> MDSKHQCVKLNDGHFMPVLGFGTYAPPEVPRSKALEVTKLAIEAGFRHIDSAHLYNNEEQVGLAIRSKIADGSVKREDIFYTSKLWSTFHRPELVRPALENSLKKAQLDYVDLYLIHSPMSLKPGEELSPTDENGKVIFDIVDLCTTWEAMEKCKDAGLAKSIGVSNFNRRQLEMILNKPGLKYKPVCNQVECHPYFNRSKLLDFCKSKDIVLVAYSALGSQRDKRWVDPNSPVLLEDPVLCALAKKHKRTPALIALRYQLQRGVVVLAKSYNEQRIRQNVQVFEFQLTAEDMKAIDGLDRNLHYFNSDSFASHPNYPYSDEYLEHHHHHH

Aldo-keto reductase 1C3 (AKR1C3; also known as prostaglandin F synthase, type 5 17β-hydroxysteroid dehydrogenase, type 2 3α-hydroxysteroid dehydrogenase, and dihydrodiol dehydrogenase X) is a human enzyme that catalyses the reduction of carbonyl groups on both steroids and prostaglandins. The enzyme forms an α8β8 barrel structure with a large and multi-cavity active site that exhibits flexibility at both the level of individual side chains as well as entire loop regions upon ligand binding. The active site contains a conserved catalytic tetrad consisting of H117-Y55-K84-D50 with Tyr-55 acting as a general acid and base, as well as the oxidised cofactor, NADP+, deep in the site. Non-steroidal anti-inflammatory drugs (NSAIDs) have been well characterised as potent AKR1C3 inhibitors.

Naproxen deviates most from the core structure in that it contains a fused 2 ring system and is then best described as a 6-methoxynaphthalene derivative. We determined the structures of flurbiprofen, ibuprofen, and naproxen bound to the AKR1C3 protein at 2.0, 1.8, and 1.9 Å respectively. In each case, a racemic mixture of R- and S-enantiomer was soaked into preformed protein crystals. In all three structures the protein selects the R-enantiomer, the opposite enantiomer to that which binds COX-1 and COX-2. The naproxen structure is unique in having a disordered cryoprotectant ethylene glycol molecule occupy the SP3 pocket – this location in the other two structures contains conserved water molecules that overlay the ethylene glycol molecule closely. The naproxen active site also contains an ethylene glycol molecule located similarly to the organic solvent molecules of flufenamic and mefenamic acid structures. A detailed comparison of (R)- and (S)-naproxen AKR1C3 complexes shows subtle differences in the protein-ligand contacts in each system. The (S)-naproxen molecule displays 86 protein ligand contacts with 8 active site side chains and the NADP molecule, while (R)-naproxen makes fewer contacts at 78 but with 12 active site side chains and NADP. These intermolecular interactions translate to different percentages of the ligand surfaces in contact with the active site; (S)-naproxen shows a 384 Å2 complementary surface with the protein out of a theoretical 429 Å2, or 90% complementarity, while (R)-naproxen shows greater complementarity of 95% which might explain the subtle preference of AKR1C3 for the R-stereoisomer we observe in our crystallographic experiments. An additional active site protrusion in AKR1C1 and 1C2 is His-222 - the site in our (R)-naproxen structure occupied by an ethylene glycol molecule.> MAIYADNSYSIGNTPLVRLKHFGHNGNVVVKIEGRNPSYSVKCRIGANMVWQ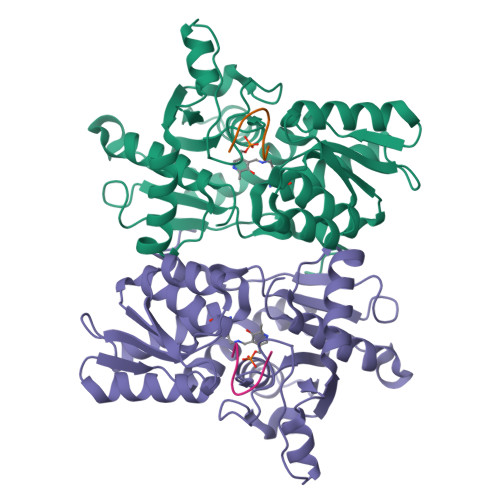AEKDGTLTKGKEIVEPTSGNTGIALAYVAAARGYKITLTMPETMSIERKRLLCGLGVNLVLTEGAKGMKGAIAKAEEIVASDPSRYVMLKQFENPANPQIHRETTGPEIWKDTDGKVDVVVAGVGTGGSITGISRAIKLDFGKQITSVAVEPVESPVISQTLAGEEVKPGPHKIQGIGAGFIPKNLDLSIIDRVETVDSDTALATARRLMAEEGILAGISSGAAVAAADRLAKLPEFADKLIVVILPSSSERYLSTALFEGIEG;> IGDGYEFT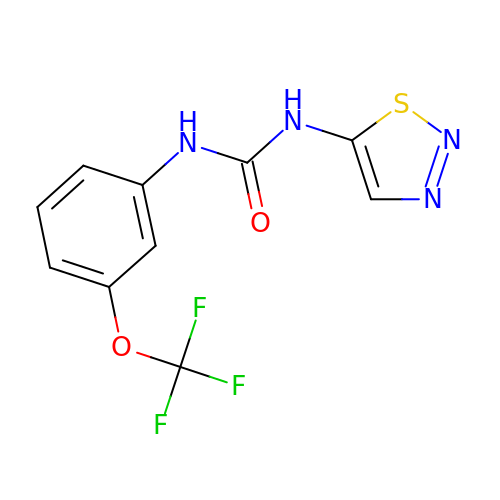1-(1,2,3-thiadiazol-5-yl)-3-[3-(trifluoromethoxy)phenyl]urea | C10 H7 F3 N4 O2 S | CKHACPXJTNTCBW-UHFFFAOYSA-N>[2x]G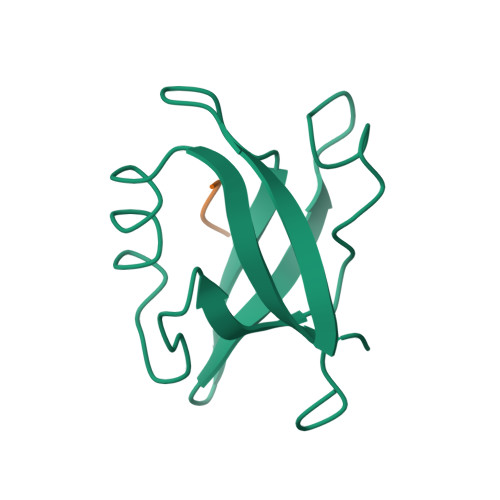PLGSKIVRIEKARDIPLGATVRNEMDSVIISRIVKGGAAEKSGLLHEGDEVLEINGIEIRGKDVNEVFDLLSDMHGTLTFVLIPSQ;>[2x]EGVPDLLV> MDFSPINCLIFALDDTLYPLKTGIAPAVKKNIDDFLVEKFGFSESKASSLRVELFKTYGSTLAGLRALGHDVHPDEYHSFVHGRLPYGSIEPNNKLRNLLNKIKQRKIIFTNSDKNHAVKVLKKLGLEDCFEEMICFETMNPNLFGSTTRPDEYPVVLKPSLTAMDICIRVANVDPRRTVFLDDNIHNITAGKSVGLRTILVGRAEKTKDADYAVETVT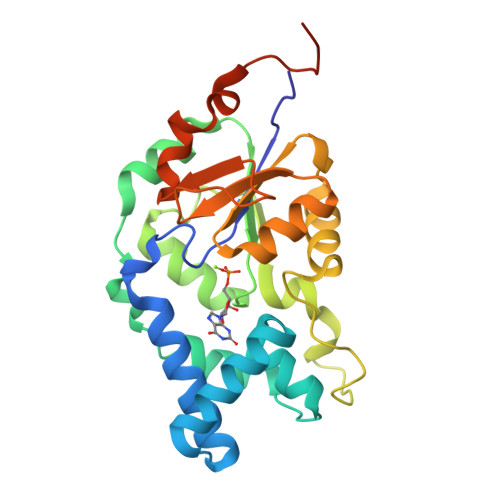EIATAVPEIWATATATGGFDVGGERIRRSKS5-chloro-2-fluoro-N-[1-(4-piperidyl)pyrazol-4-yl]benzenesulfonamide 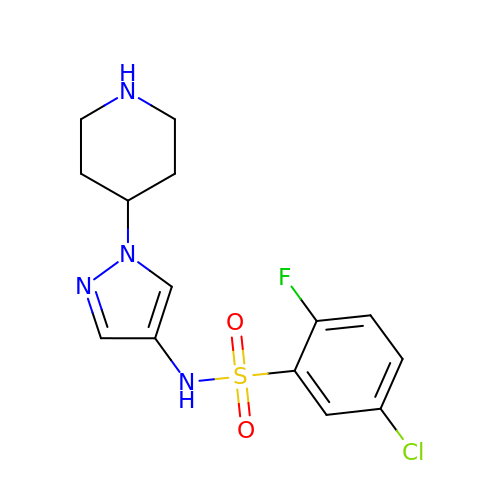| C14 H16 Cl F N4 O2 S | XMUAZEINLRUFHP-UHFFFAOYSA-N>[2x]MNVGIKGFGAYAPEKIIDNAYFEQFLDTSDEWISKM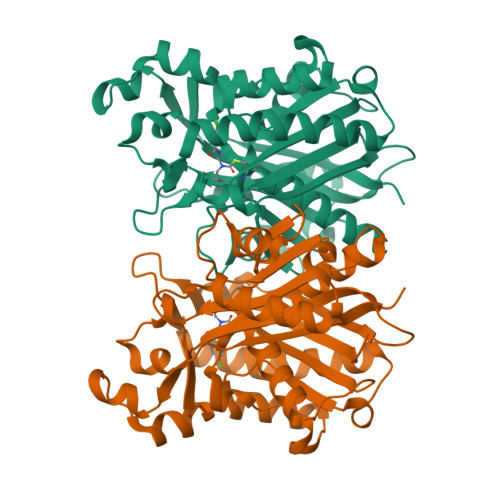TGIKERHWADDDQDTSDLAYEASVKAIADAGIQPEDIDMIIVATATGDMPFPTVANMLQERLGTGKVASMDQLAACSGFMYSMITAKQYVQSGDYHNILVVGADKLSKITDLTDRSTAVLFGDGAGAVIIGEVSEGRGIISYEMGSDGTGGKHLYLDKDTGKLKMNGREVFKFAVRIMGDASTRVVEKANLTSDDIDLFIPHQANIRIMESARERLGISKDKMSVSVNKYGNTSAASIPLSIDQELKNGKLKDDDTIVLVGFGGGLTWGAMTIKWGK2-methylbuta-1,3-diene | C5 H8 | 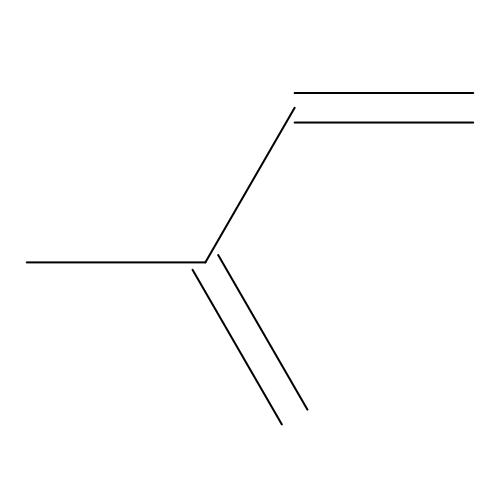RRHGJUQNOFWUDK-UHFFFAOYSA-N> IVGGKVCPKGECPWQVLLLVNGAQLCGGTLINTIWVVSAAHCFDKIKNWRNLIAVLGEHDLSEHDGDEQSRRVAQVIIPSTYVPGTTNHDIALLRLHQPVVLTDHVVPLCLPERTFSERTLAFVRFSLVSGWGQLLDRGATALELMVLNVPRLMTQDCLQQSRKVGDSPNITEYMFCAGYSDGSKDSCKGDSGGPHATHYRGTWYLTGIVSWGQGCATVGHFGVYTRVSQYIEWLQKLMRSEPRPGVLLRAPFP;> ANAFLEELRPGSLERECKEEQCSFEEAREIFKDAERTKLFWISYSDGDQCASSPCQNGGSCKDQLQSYICFCLPAFEGRNCETHKDDQLICVNENGGCEQYCSDHTGTKRSCRCHEGYSLLADGVSCTPTVEYPCGKIPILE;> TVAAYNLTWKSTNFKTILEWEPKPVNQVYTVQISTKSGDWKSKCFYTTDTECDLTDEIVKDVKQTYLARVFSYPA;> EPLYENSPEFTPYLETNLGQPTIQSFEQVGTKVNVTVEDERTLVRRNNTFLSLRDVFGKDLIYTLYYWSGKKTAKTNTNEFLIDVDKGENY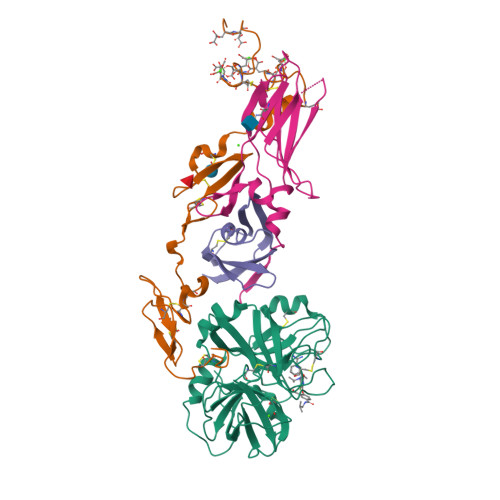CFSVQAVIPSRTVNRKSTDSPVECM4-[4-[(4,4-dimethylpiperidin-1-yl)methyl]phenyl]-9-(7H-pyrrolo[2,3-d]pyrimidin-4-yl)-1,4,9-triazaspiro[5.5]undecan-2-one 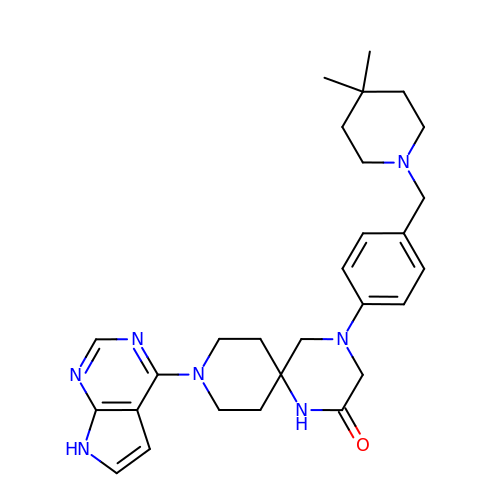| C28 H37 N7 O | BJJFIFKPWWSNGM-UHFFFAOYSA-N Kinesins constitute a superfamily of microtubule-based motor proteins with important cellular functions ranging from intracellular transport to cell division. In the early stages of mitosis, during prometaphase, certain kinesins are required for the formation of the bipolar spindle, such as Eg5 and Kif15, which seem to possess partially overlapping functions. Kif15 has recently come to the fore because it can substitute the functions of Eg5, and may itself have potential as a prospective drug target. In contrast, Kif15 works as a dimer by crosslinking parallel kinetochore-MTs and we demonstrated that it does not contain an MT-binding site within its tail domain.

The structure of the Kif15 motor domain was solved by molecular replacement and refined to a resolution of 2.7 Å. Kif1519–375 crystallized in space group P3221 with three molecules in the asymmetric unit. The final model contains residues 24–375 for molecules A and B and residues 24–372 for molecule C. Owing to missing or non-interpretable electron density, several smaller loops could not be built and are absent from the model. Since molecule A presented better defined electron density and a more complete model than molecules B and C, we subsequently use it for further descriptions of the structure. The crystallized Kif15 construct contains the neck linker, which aligns with the catalytic core, forming a small β-sheet. Although Mg2+-ADP is bound in the catalytic site, Kif15 is in the so-called ‘ATP-like’ conformation. Although Kif15 contains ADP in the catalytic site, its motor-domain structure was captured in the ‘ATP-like’ configuration, with the neck linker docked to the catalytic core. Loop L11 is not visible in any of the three molecules in the asymmetric unit. In Eg5, loop L5 is known to be important for inhibitor binding, and differences in the length of this motif in Kif15 (in Kif15 this loop is shorter) explain why Eg5-targeting inhibitors do not inhibit Kif15. In addition, several other key residues involved in inhibitor binding in Eg5, such as Glu116, Arg119, Trp127 and Ala216, are not present in Kif15.

>[3x]GAMGQPSNEGDAIKVFVRIRPPAERSGSADGEQNLCLSVLSSTSLRLHSNPEPKTFTFDHVADVDTTQESVFATVAKSIVESCMSGYNGTIFAYGQTGSGKTFTMMGPSESDNFSHNLRGVIPRSFEYLFSLIDREKEKAGAGKSFLCKCSFIEIYNEQIYDLLDSASAGLYLREHIKKGVFVVGAVEQVVTSAAEAYQVLSGGWRNRRVASTSMNRESSRSHAVFTITIESMEKSNEIVNIRTSLLNLVDLAGSERQKDTHAEGMRLKEAGNINRSLSCLGQVITALVDVGNGKQRHVCYRDSKLTFLLRDSLGGNAKTAIIANVHPGSRCFGETLSTLNFAQRAKLIKNKAVVNEDTQG> MKVPVMMADESIATINHPEDDWKIWTVINPATWMVPFFGILFVQMWLIHSYALSLPGYGFKDSV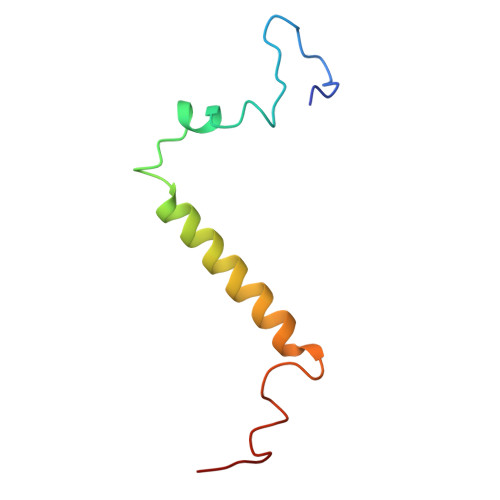RVAQPA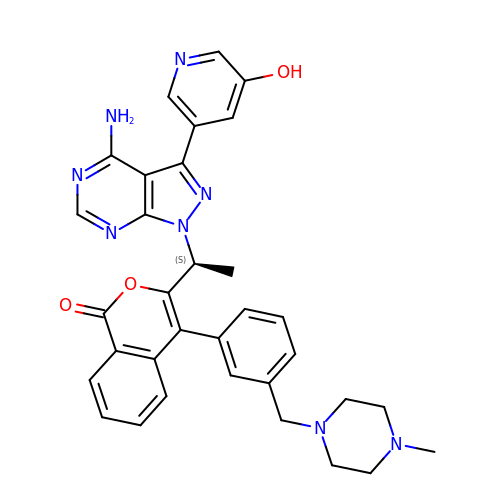3-[(1S)-1-[4-azanyl-3-(5-oxidanylpyridin-3-yl)pyrazolo[3,4-d]pyrimidin-1-yl]ethyl]-4-[3-[(4-methylpiperazin-1-yl)methyl]phenyl]isochromen-1-one | C33 H32 N8 O3 | JSUNXOYZTNBLOP-FQEVSTJZSA-N Chaperone-Usher Pathway (CUP) pili are among the most widely distributed and best-characterized adhesins in Gram-negative bacteria. In the assembled pilus, each pilin subunit provides its N-terminal β-strand to the following subunit to complete its Ig-like fold in a process termed donor-strand complementation. The best-characterized archaic CUP pili include the CupE system in P. aeruginosa and the Csu system in Acinetobacter baumannii. Archaic CUP pili are crucial for the formation of biofilms, which play an important role in persistent and chronic infections.

After deducing the symmetry of the pilus from two-dimensional class averages of single filaments, we performed helical reconstruction and obtained a 3.5 Å-resolution cryo-EM density, from which an atomic model of the CupE pilus could be built. The atomic model reveals an arrangement of CupE1 subunits in a zigzag architecture (215° right-handed rotation per subunit). In agreement with classical CUP proteins, the N-terminal β1-strand of each (n+1)th subunit completes the Ig-like fold of the nth subunit. This donor strand interacts with the nth subunit through both β-sheet hydrogen bonding as well as hydrophobic interactions, filling a hydrophobic groove in the subunit core. The structure also shows two key cysteine residues (C41-C85) forming a disulfide bridge within a β-sheet from which the donor strand extends. The 13-residue donor strand of the (n+1)th subunit represents the majority of the interaction with the nth subunit. The interface between the Ig-like domains is relatively small in comparison to the extensive donor-strand interactions, and is mainly maintained by the interaction of a loop with the next subunit, with two interacting valine residues V69 and V48 at the core of the interaction. Thus, the CupE pilus shows a relaxed arrangement of subunits compared to the tight packing of the Csu pilus, resulting in a higher rise per subunit than in the Csu pilus. Visual inspection of the CupE pilus along the helical axis showed a serine and threonine-rich loop (TTTTSST) extending outward from the helical axis of the CupE pilus, constituting the part of the subunit that is most exposed to the environment. In the EM map, we noticed extra density near the loop that could not be attributed to the atomic model of the CupE1 protein subunit and that we suspected might correspond to a post-translational modification.

>AGTLIGQVGVQMVIGAGCTIINGSVSGGINQWGTLDFGSHSDLTNVVDAQTVGTSGNIQIQCSTGLTPSLTVNAGLHASGGQRYMQNTTTTSSTIAYNIYSDAARSALIQANTPVDISSVSTGTAVNIPLYGRVVPTGQSTPTPTAGTYTDTLLVTIAW[5x]>CCCCGCGGGG[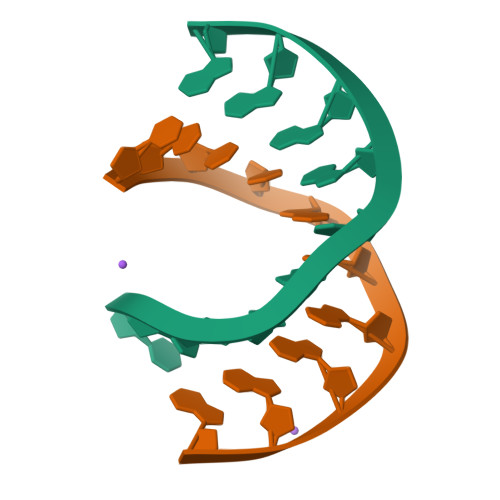2x]3-[(1S)-1-(DIMETHYLAMINO)ETHYL]PHENOL | C10 H15 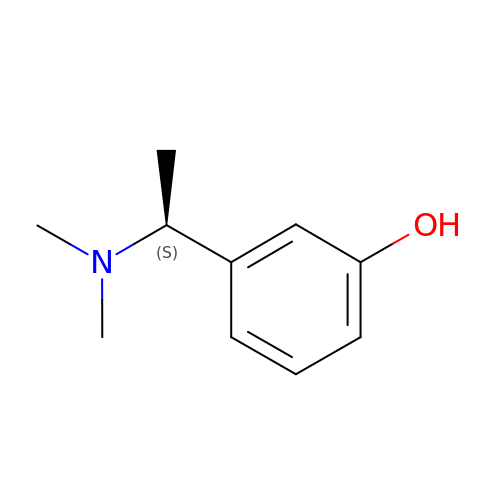N O | GQZXRLWUYONVCP-QMMMGPOBSA-N> AEAWYNLGNAYYKQGDYDEAIEYYQKALELDPRSAEAWYNLGNAYYKQGDYDEAIEYYQKALELDPRSAEAWYNLGNAYYKQGDYDEAIEYYQKALELDPRSAEAWYNLG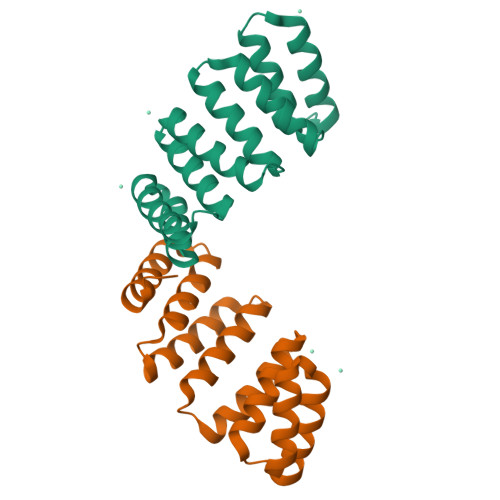NAYYKQGDYDEAIEYYQKALELDPRS> MHISDEQLKRPLRDYGEALEMWSTFQTKTQALSQSLSSQLRLILTGSGIPSKRAYQILLCVDDSSSMSDDNRSTAGNLALESLVMVARALTVLEAGQIGVMGFGTDVFVAHALTDPPFTSQDAGARVLQQFTFRQDSTDMVLLLRRTIDHFREARLIQASSSRGGEDLWQLALILSDGLVQSRDHARLR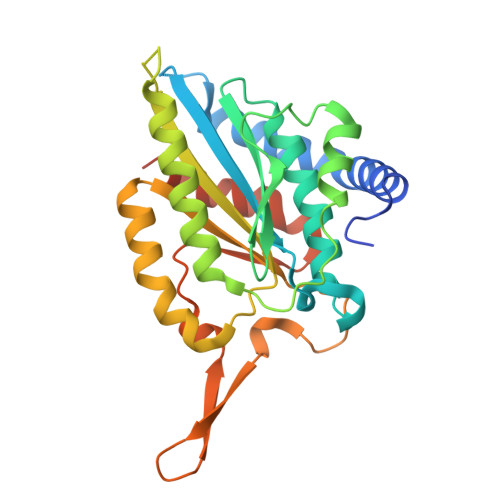PLLREAMEQRVMVVFIVMDDARSRKGHSVLELKEARFGPDGVPVIHRYLDSFPFPYYLIVHHLEDLPGALAALLRTWFAEVNSGSHHHHHH>MEISQPSIGIFYISKVLALAPYATVRNSKGRVEIGRSWLFTVYSATLTVVMVFLTYRGLLFDANSEIPVRMKSATSKVVTALDVSVVVMAIVSGVYCGLFSLNDTLELNDRLNKIDNTLNAYNNFRRDRWRALGMAAVSLLAISILVGLDVGTWMRIAQDMNIAQSDTELNVHWYIPFYSLYFILTGLQVNIANTAYGLGRRFGRLNRMLSSSFLAENNATSAIKPQKVSTVKNVSVNRPAMPSALHASLTKLNGETLPSEAAAKNKGLLLKSLADSHESLGKCVHLLSNSFGIAVLFILVSCLLHLVATAYFLFLELLSKRDNGYLWVQMLWICFHFLRLLMVVEPCHLAARESRKTIQIVCEIERKVHEPILAEAVKKFWQQLLVVDADFSACGLCRVNRTILTSFASAIATYLVILIQFQRTNGLEGGSSGGWSHP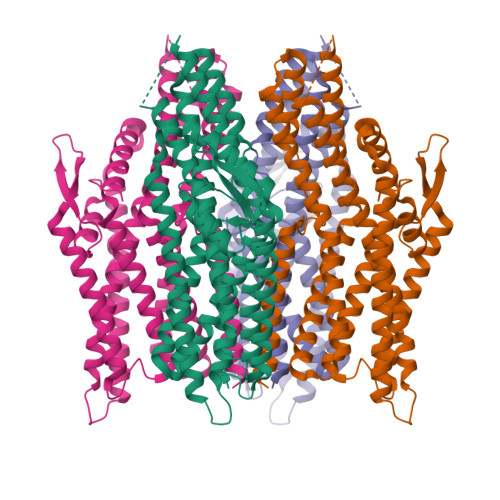QFEK[4x]>[2x]GPGVCKSYKSVALVVGVTGIVGSSLAEVLKLPDTPGGPWKVYGVARRPCPVWLAKKPVEYIQCDVSNNQETISKLSPLKDITHIFYVSWIGSEDCQTNATMFKNILNSVIPNASNLQHVCLQTGIKHYFGIFEEGSKVVPHDSPFTEDLPRLNVPNFYHDLEDILYEETGKNNLTWSVHRPALVFGFSPCSMMNIVSTLCVYATICKHENKALVYPGSKNSWNCYADAVDADLVAEHEIWAAVDP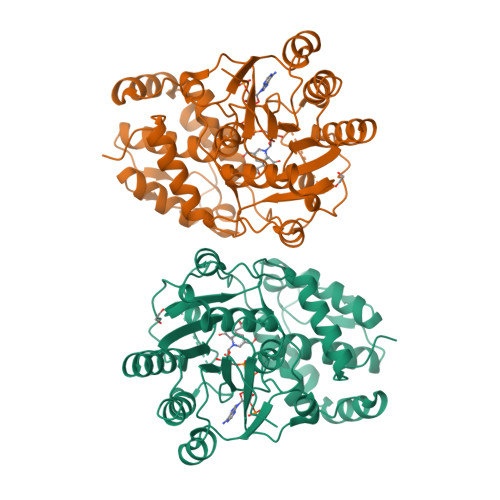KAKNQVLNCNNGDVFKWKHIWKKLAEEFGIEMVGYVEGKEQVSLAELMKDKDQVWDEIVKKNNLVPTKLKEIAAFWFADIAFCSENLISSMNKSKELGFLGFRNSMKSFVSCIDKMRDYRFIPKAF> MDYN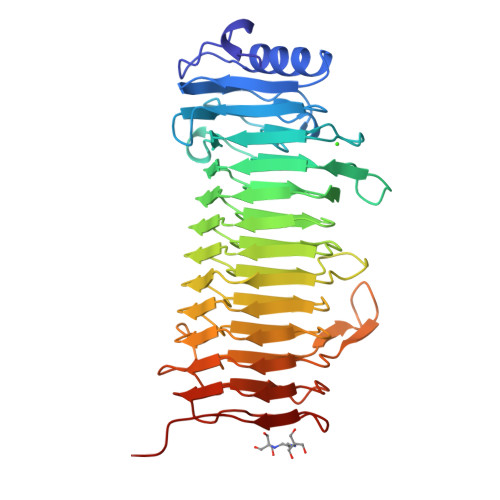VKDFGALGDGVSDDRVAIQAAIDAAHAAGGGTVYLPPGEYRVSAAGEPSDGCLTLRDNVYLAGAGMGQTVIKLVDGSAQKITGIVRSPFGEETSNFGMRDLTLDGNRANTVDKVDGWFNGYAPGQPGADRNVTIERVEVREMSGYGFDPHEQTINLVLRDSVAHHNGLDGFVADYQIGGTFENNVAYANDRHGFNIVTSTNDFVMRNNVAYGNGGNGLVVQRGSENLAHPENILIDGGSYYDNGLEGVLVKMSNNVTVQNADIHGNGSSGVRVYGAQGVQILGNQIHDNAKTAVAPEVLLQSYDDTLGVSGNYYTTLNTRVEGNTITGSANSTYGVQERNDGTDFSSLVGNTINGVQEAAHLYGPNSTVSGTVSAPPQGTDLE By incorporating a light‐responsive protein domain into HaloTag, we engineer a tunable, photoswitchable HaloTag (psHaloTag), which can reversibly modulate the fluorescence of a bound dye‐ligand via a light‐induced conformational change. As the genetically encoded photoswitch, we selected the light‐oxygen‐voltage 2 domain of Avena sativa phototropin 1 (AsLOV2). Exposure to 450 nm light induces the formation of a metastable photo‐adduct between a cysteine side chain and the FMN cofactor, which leads to structural rearrangements and undocking and unfolding of the Jα helix. Upon illumination, the conformational change of the protein photoswitch alters the dye environment, shifting its equilibrium towards the open, fluorescent state.

The crystals formed in space group C121 and contained two assemblies per asymmetric unit. The two psHaloTag1a molecules adopt a near‐identical conformation with a root‐mean‐square deviation (RMSD) of 0.33 Å (for 431 Cα residues). The extended Jα helix is in a folded state in both molecules and consists of about 1/3 HaloTag and 2/3 LOV domain residues. The FMN cofactors, JF635‐HTL fluorophore ligands, and Cl− ions were clearly visible in the electron density. Based on the density, both FMN molecules appear to be unbound to the adjacent C189 residues, and the folded helix of the LOV domain suggests crystallization of the OFF state. JF635‐HTL adopted the same position as analogous fluorophore ligands on HaloTag, and while the electron density around the dyes does not allow for unambiguous identification of the open or closed conformation, the open conformation resulted in the best fit. While we would expect a primarily closed conformation in solution for the OFF state, the observed open form could be explained by the tight crystal packing around the fluorophore, as the surface‐exposed dyes from the two chains face each other in the center of the asymmetric unit. The two performance‐increasing mutations E143W and A285W are in proximity to each other, and A285W to the headgroup of the JF635‐HTL fluorophore. These tryptophane residues could form an extended hydrophobic network together with neighboring hydrophobic residues (I150, L147, and additional residues towards the center of the protein), which could improve the stabilization/interaction of the fluorophore and improve performance. Overall, both the predicted and the crystal structures show that the HaloTag and LOV domains are tightly arranged and connected by a long helix, which ensures efficient propagation of the conformational change to the HaloTag in close proximity to the fluorophore.

>[2x]GPMAEIGTGFPFDPHYVEVLGERMHYVDVGPRDGTPVLFLHGNPTSSYVWRNIIPHVAPTHRCIAPDLIGMGKSDKPDLGYFFDDHVRFMDAFIEALGLEEVVLVIHDWGSALGFHWAKRNPERVKGIAFMEFIRPIPTWDEWPWFAGLERIEKNFIITDPRLPDNPIIFASDSFLQLTEYSREEILGRNCRFLQGPETDRATVRKIRDAIDNQTEVTVQLINYTKSGKKFWNLFHLQPMRDQKGDVQYFIGVQLDGTEHVRDAAEREGVMLIKKTAENIDEAAPFWRETFQAFRTTDVGRKLIIDQNVFIEGTLPMGVVRPLTEVEMDHYREPFLNPVDREPLWRFPNELPIAGEPANIVALVEEYMDWLHQSPVPKLLFWGTPGVLIPPAEAARLAKSLPNCKAVDIGPGLNLLQEDNPDLIGSEIARWLSTLEISG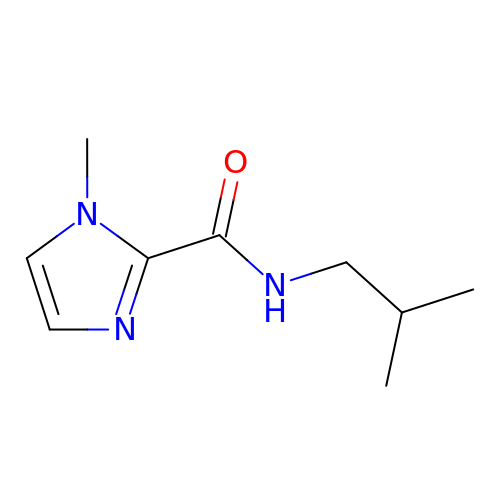1-methyl-N-(2-methylpropyl)-1H-imidazole-2-carboxamide | C9 H15 N3 O | ITOJSUFSGQMSOE-UHFFFAOYSA-N3-METHYLCYTOSINE | C5 H8 N3 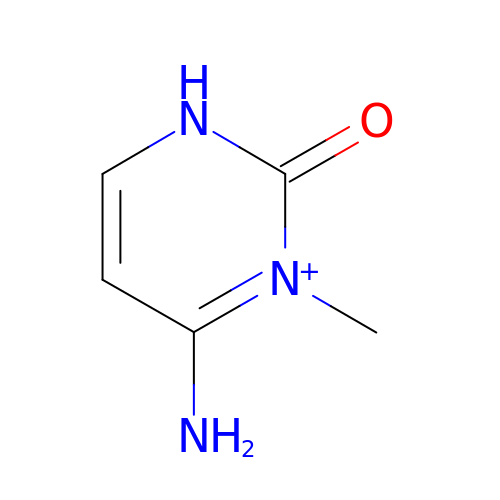O | UPHQQDZIRIHPHU-UHFFFAOYSA-O> MYTREELMEIVSERVKKCTACPLHLNRTNV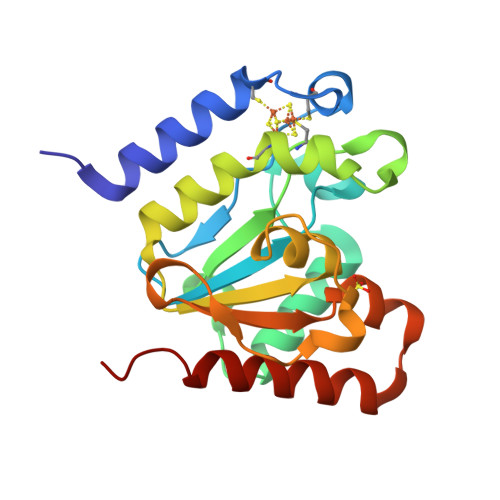VVGEGNLDTRIVFVGEGPGEEEDKTGRPFVGRAGMLLTELLRESGIRREDVYICNVVKCRPPNNRTPTPEEQAACGHFLLAQIEIINPDVIVALGATALSFFVDGKKVSITKVRGNPIDWLGGKKVIPTFHPSYLLRNRSNELRRIVLEDIEKAKSFIKKEG>MAQILPIRFQEHLQLQNLGINPANIGFSTLTMESDKFICIREKVGEQAQVVIIDMNDPSNPIRRPISADSAIMNPASKVIALKAGKTLQIFNIEMKSKMKAHTMTDDVTFWKWISLNTVALVTDNAVYHWSMEGESQPVKMFDRHSSLAGCQIINYRTDAKQKWLLLTGISAQQNRVVGAMQLYSVDRKVSQPIEGHAASFAQFKMEGNAEESTLFCFAVRGQAGGKLHIIEVGTPPTGNQPFPKKAVDVFFPPEAQNDFPVAMQISEKHDVVFLITKYGYIHLYDLETGTCIYMNRISGETIFVTAPHEATAGIIGVNRKGQVLSVCVEEENIIPYITNVLQNPDLALRMAVR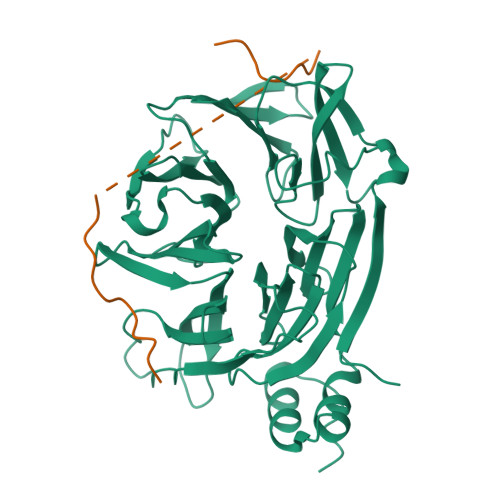NNLAGAEELF[4x];>LAVTPDAASQPLIDLPLIDFCDTPEAHVAVGSESRPLIDLMTNTPDMNKNVAKPSPVVGQLIDLSSP[4x]> MAAIPALDPEAEPSMDVILVGSSELSSSVSPGTGRDLIAYEVKANQRNIEDICICCGSLQVHTQHPLFEGGICAPCKDKFLDALFLYDDDGYQSYCSICCSGETLLICGNPDCTRCYCFECVDSLVGPGTSGKVHAMSNWVCYLCLPSSRSGLLQRRRKWRSQLKAFYDRESENPLEMFETVPVWRRQPVRVLSLFEDIKKELTSLGFLESGSDPGQ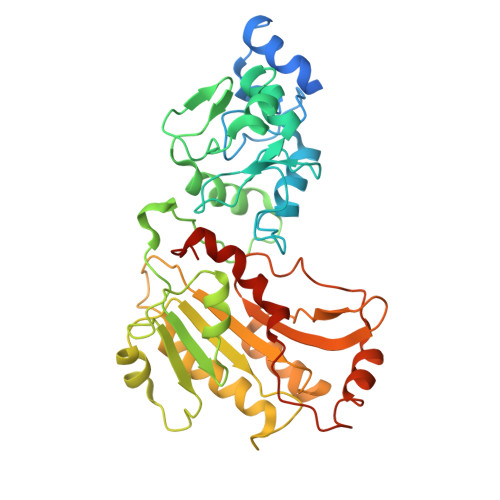LKHVVDVTDTVRKDVEEWGPFDLVYGATPPLGHTCDRPPSWYLFQFHRLLQYARPKPGSPGPFFWMFVDNLVLNKEDLDVASRFLEMEPVTIPDVHGGSLQNAVRVWSNIPAIRSRHWALVSEEELSLLAQNKQSSKLAAKWPTKLVKNCFLPLREYFKYFSTELTSSL>MTDTPFIRPDMKAFLEAIAAMAGPTLAEMTLEEARASYVALHGMADRPARELAVIRNLSCPGPAGDIPLRLYDARESREAGPVITFYHGGGFVIGDLDTHHNLCTEIAALMDLPVVAVDYRLAPEHPFPAAIEDCEAATRWVASSPSELGRTASGVIPIGDSAGGNATIVVSQLLGAKPADVPVVLQVPIFPLASDAVGSASLEAFAEGFVLTKASIEFFDTAYKADRADPRGFPILGDHTAAPPTIVATASLDPIRDSGRDYAKALVEAGRDVVYLEMEGVTHSFTNIRAAVPSTQGDLERIIAAMKMMLGTA[3x];> MTDTPFIRPDMKAFLEAIAAMAGPTLAEMTLEEARASYVALHGMADRPARELAVIRNLSCPGPAGDIPLRLYDARESREAGPVITFYHGGGFVIGDLDTHHNLCTEIAALMDLPVVAVDYRLAPEHPFPAAIEDCEAATRWVASSPSELGRTASGVIPIGDSAGGNATIVVSQLLGAKPADVPVVLQVPIFPLASDAVGSASLAAFAEGFVLTKASIEFFDTAYKADRADPRGFPILGDHTAAPPTIVATASLDPIRDSGRDYAKALVEAGRDVVYLEMEGVTHSFTNIRAAVPSTQGDLERIIAAMKMMLGTA

To advance the understanding of esterases, we have identified and characterized E53, an alkalophilic esterase from a marine bacterium Erythrobacter longus. Family IV esterases, to which E53 belongs, are widely distributed in microorganisms, plants, and animals, specifically degrade short-chain esters. The family IV esterase can be characterized by the α/β-fold hydrolase group, and contains two distinct structural domains: an N-terminal CAP domain and a C-terminal catalytic domain. The catalytic reaction relies on the S-H-D/E catalytic triad located in the catalytic domain.

The WT E53 with 314 amino acids has a typical α/β-hydrolase fold. It contains eight β-strand and nine α-helices. Two α-helices (α1 and α2) at the N-terminal region form a CAP domain, the conserved domain present in all microbial family IV esterases. The catalytic triad was composed of S162, D254, and H284. The oxyanion hole was composed of G90 and G91 within the conserved HGGG motif (amino acids No. 88-91). In order to describe the catalytic pocket in a concise way, three regions were defined: R1—catalytic center region, R2—pocket entrance channel area and R3—end area of pocket. The C6 substrate was modeled based on the electron density at the catalytic center of the pocket between the oxyanion hole (G90 and G91) and two residues of the catalytic triad (S162 and H284). The p-NP substrate was accommodated in the R3 region while the carboxyl acid was pointing in the direction of the pocket entrance. In the R2 region, the crystal structure of the WT E53 exhibits a structural bottleneck close to the entrance of the pocket, determined by V211 and S216. The hydrogen bond established via the side chain from asparagine with the amino acids L193 (2.9 Å between the amide and carbonyl oxygen) and G233 (3.0 Å between the amide and carbonyl oxygen) may contribute to the stability of the enzyme under the alkaline condition.> MINMARFDKKETIRTMTDTGLVPVFCSCDVEVAKQVIRACYNGGVRVFEFTNREEAAHEVFGAVSRWIVEACPEMILGVGSIVDAPTASLYLQSGANFVVGPLTNPDIAKVCNRRLVPYIPGCGSVSEVGYAQELGCDICKVFPGDVLGPGFVKALKAPMPWSQVMVTGGVKPKEANLKAWFDAGATCVGMGSNLFPPEAIASGNWEKITDICAQALGVIREVRKE

Chondroitin sulfate A is a linear, sulfated carbohydrate linked to periodontal disease as the principal species of glycosaminoglycan appended on the surface of cortical bone of teeth and in supporting dental ligaments. Through genomic comparisons with B. thetaiotaomicron, a new PUL-like operon (Bfo2285-Bfo2295, and Bfo3043) was identified in T. forsythia and the crystal structure of two proteins from this PUL-like operon, Bfo2290 and Bfo2294, were reported using X-ray crystallography. Here we define a pathway for the degradation of CSA by T. forsythia based on the discovery of a PUL-like gene cluster found using bioinformatics analysis, functionally characterize three proteins (Bfo2285, Bfo2290, Bfo2291, and Bfo2294) from this PUL-like gene cluster and report the crystal structure of an exo-N-acetylgalactosamine (Bfo2290) and for a 2-keto-3-deoxy-6-phosphogluconate (KDPG) and 2-keto-4-hydroxyglutarate (KHP) to D-glyceraldehyde-3-phosphate aldolase (Bfo2294). As CSA is the primary GAG in alveolar bone, this likely serves as a mechanism by which T. Forsythia compromises periodontal tissues contributing to bone loss in periodontal disease in conjunction with host osteoclastic activity.

The structure of Bfo2294 was solved to a resolution of 2.20Å in the space group of P23 and iteratively built and refined to a corresponding Rwork of 0.179 and Rfree of 0.221. Bfo2294 was found to have an α/β-barrel structure and contained a glutamic acid and lysine zwitterionic-pair typical of class I aldolases which use a Schiff-base mechanism to convert KDPG and KHP into D-glyceraldehyde-3-phosphate and pyruvate. Key residues highlighted in yellow Glu 49 and Lys 141 form a zwitterionic-pair critical to the catalytic function of Bfo2294. KDP was modeled in orange as part of the co-crystal structure of a KDPGal aldolase to show the orientation of the substrate in the active site. Enzyme kinetic studies previously conducted by Eshaque et al. was successful in showing that Bfo2294 is a KDPG aldolase. As the enzyme was found to be dependent on NADH as a cofactor, the enzyme kinetic constants of Bfo2294 were determined by quantifying the decrease in concentration of NADH by measuring the decrease in absorbance at 340nm as it was consumed in the reaction. Analysis of substrate specificity and pH optimization by Eshaque et al. also showed that the preferred substrate for Bfo2294 was CSA at pH 6.5. The assay was not repeated for KHG, however through multiple sequence alignments and comparisons against structural homologs, Bfo2294 may also be capable of similarly degrading KHG.>MRIILLGAPGAGKGTQAQFIMEKYGIPQISTGDMLRAAVKSGSELGKQAKDIMDCGKLVTDELVIALVKERIAQEDSRNGFLLDGFPRTIPQADAMKEAGINVDYVLEFDVPDELIVDRIVGRRVHAPSGRVYHVKFNPPKVEGKDDVTGEELTTRKDDQEETVRKRLCEYHQMTAPLIGYYSK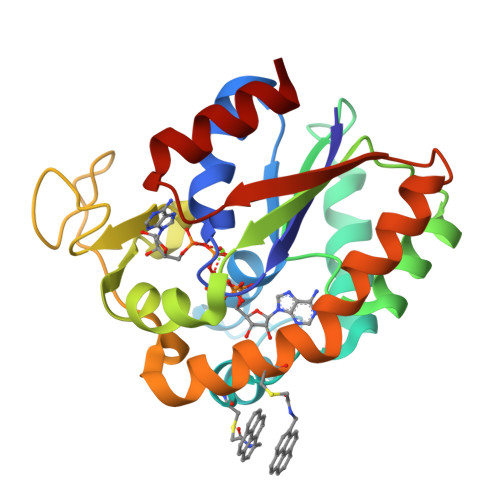EAEAGNTKYAKVDGTKPVAEVRADLEKILG[2x]>MPSSLLGAAMPASTSAAALQEALENAGRLIDRQLQEDRMYPDLSELLMVSAPNNPTVSGMSDMDYPLQGPGLLSVPNLPEISSIRRVPLPPELVEQFGHMQCNCMMGVFPPISRAWLTIDSDIFMWNYEDGGDLAYFDGLSETILAVGLVKPKAGIFQPHVRHLLVLATPVDIVILGLSYANLQTGSGVLNDSLSGGMQLLPDPLYSLPTDNTYLLTITSTDNGRIFLAGKDGCLYEVAYQAEAGWFSQRCRKINHSKSSLSFLVPSLLQFTFSEDDPILQIAIDNSRNILYTRSEKGVIQVYDLGQDGQGMSRVASVSQNAIVSAAGNIARTIDRSVFKPIVQIAVIENSESLDCQLLAVTHAGVRLYFSTCPFRQPLARPNTLTLVHVRLPPGFSASSTVEKPSKVHRALYSKGILLMAASENEDNDILWCVNHDTFPFQKPMMETQMTAGVDGHSWALSAIDELKVDKIITPLNKDHIPITDSPVVVQQHMLPPKKFVLLSAQGSLMFHKLRPVDQLRHLLVSNVGGDGEEIERFFKLHQEDQACATCLILACSTAACDREVSAWATRAFFRYGGEAQMRFPTTLPPPSNVGPILGSPVYSSSPVPSGSPYPNPSFLGTPSHGIQPPAMSTPVCALGNPATQATNMSCVTGPEIVYSGKHNGICIYFSRIMGNIWDASLVVERIFKSGNREITAIESSVPCQLLESVLQELKGLQEFLDRNSQFAGGPLGNPNTTAKVQQRLIGFMRPENGNPQQMQQELQRKFHEAQLSEKISLQAIQQLVRKSYQALALWKLLCEHQFTIIVAELQKELQEQLKITTFKDLVIRDKELTGALIASLINCYIRDNAAVDGISLHLQDICPLLYSTDDAICSKANELLQRSRQVQNKTEKERMLRESLKEYQKISNQVDLSNVCAQYRQVRFYEGVVELSLTAAEKKDPQGLGLHFYKHGEPEEDIVGLQAFQERLNSYKCITDTLQELVNQSKAAPQSPSVPKKPGPPVLSSDPNMLSNEEAGHHFEQMLKLSQRSKDELFSIALYNWLIQVDLADKLLQVASPFLEPHLVRMAKVDQNRVRYMDLLWRYYEKNRSFSNAARVLSRLADMHSTEISLQQRLEYIARAILSAKSSTAISSIAADGEFLHELEEKMEVARIQLQIQETLQRQYSHHSSVQDAVSQLDSELMDITKLYGEFADPFKLAECKLAIIHCAGYSDPILVQTLWQDIIEKELSDSVTLSSSDRMHALSLKIVLLGKIYAGTPRFFPLDFIVQFLEQQVCTLNWDVGFVIQTMNEIGVPLPRLLEVYDQLFKSRDPFWNRMKKPLHLLDCIHVLLIRYVENPSQVLNCERRRFTNLCLDAVCGYLVELQSMSSSVAVQAITGNFKSLQAKLERLH[6x];>[4x]MDTEGFGELLQQAEQLAAETEGISELPHVERNLQEIQQAGERLRSRTLTRTSQETADVKASVLLGSRGLDISHISQRLESLSAATTFEPLEPVKDTDIQGFLKNEKDNALLSAIEESRKRTFGMAEEYHRESMLVEWEQVKQRILHTLLASGEDALDFTQESEPSYISDVGPPGRSSLDNIEMAYARQIYIYNEKIVNGHLQPNLVDLCASVAELDDKSISDMWTMVKQMTDVLLTPATDALKNRSSVEVRMEFVRQALAYLEQSYKNYTLVTVFGNLHQAQLGGVPGTYQLVRSFLNIKLPAPLPGLQDGEVEGHPVWALIYYCMRCGDLLAASQVVNRAQHQLGEFKTWFQEYMNSKDRRLSPATENKLRLHYRRALRNNTDPYKRAVYCIIGRCDVTDNQSEVADKTEDYLWLKLNQVCFDDDGTSSPQDRLTLSQFQKQLLEDYGESHFTVNQQPFLYFQVLFLTAQFEAAVAFLFRMERLRCHAVHVALVLFELKLLLKSSGQSAQLLSHEPGDPPCLRRLNFVRLLMLYTRKFESTDPREALQYFYFLRDEKDSQGENMFLRCVSELVIESREFDMILGKLENDGSRKPGVIDKFTSDTKPIINKVASVAENKGLFEEAAKLYDLAKNADKVLELMNKLLSPVVPQISAPQSNKERLKNMALSIAERYRAQGISANKFVDSTFYLLLDLITFFDEYHSGHIDRAFDIIERLKLVPLNQESVEERVAAFRNFSDEIRHNLSEVLLATMNILFTQFKRLKGTSPSSSSRPQRVIEDRDSQLRSQARTLITFAGMIPYRTSGDTNARLVQMEVLMN;>[2x]MATPLAVNSAASLWGPYKDIWHKVGNALWRRQPEAVHLLDKILKKHKPDFISLFKNPPKNVQQHEKVQKASTEGVAIQGQQGTRLLPEQLIKEAFILSDLFDIGELAAVELLLAGEHQQPHFPGLTRGLVAVLLYWDGKRCIANSLKALIQSRRGKTWTLELSPELASMTTRFTDELMEQGLTYKVLTLVSQIDVNNEFEKLQRERGLGSEKHRKEVSDLIKECRQSLAESLFAWACQSPLGKEDTLLLIGHLERVTVEANGSLDAVNLALLMALLYCFDISFIEQSTEERDDMIHQLPLLTEKQYIATIHSRLQDSQLWKLPGLQATVRLAWALALRGISQLPDVTALAEFTEADEAMAELAIADNVFLFLMESVVVSEYFYQEEFYIRRVHNLITDFLALMPMKVKQLRNRADEDARMIHMSMQMGNEPPISLRRDLEHLMLLIGELYKKNPFHLELALEYWCPTEPLQTPTIMGSYLGVAHQRPPQRQVVLSKFVRQMGDLLPPTIYIPYLKMLQGLANGPQCAHYCFSLLKVNGSSHVENIQGAGGSPVSWEHFFHSLMLYHEHLRKDLPSADSVQYRHLPSRGITQKEQDGLIAFLQLTSTIITWSENARLALCEHPQWTPVVVILGLLQCSIPPVLKAELLKTLAAFGKSPEIAASLWQSLEYTQILQTVRIPSQRQAIGIEVELNEIESRCEEYPLTRAFCQLISTLVESSFPSNLGAGLRPPGFDPYLQFLRDSVFLRFRTRAYRRAAEKWEVAEVVLEVFYKLLRDYEPQLEDFVDQFVELQGEEIIAYKPPGFSLMYHLLNESPMLELALSLLEEGVKQLDTYAPFPGKKHLEKAVQHCLALLNLTLQKENLFMDLLRESQLALIVCPLEQLLQGINPRTKKADNVVNIARYLYHGNTNPELAFESAKILCCISCNSNIQIKLVGDFTHDQSISQKLMAGFVECLDCEDAEEFVRLEEGSELEKKLVAIRHETRIHILNLLITSLECNPPNLALYLLGFELKKPVSTTNLQDPGVLGCPRTCLHAILNILEKGTEGRTGPVAVRESPQLAELCYQVIYQLCACSDTSGPTMRYLRTSQDFLFSQLQYLPFSNKEYEISMLNQMSWLMKTASIELRVTSLNRQRSHTQRLLHLLLDDMPVKPYSDGEGGIEDENRSVSGFLHFDTATKVRRKILNILDSIDFSQEIPEPLQLDFFDRAQIEQVIANCEHKNLRGQTVCNVKLLHRVLVAEVNALQGMAAIGQRPLLMEEISTVLQYVVGRNKLLQCLHAKRHALESWRQLVEIILTACPQDLIQAEDRQLIIRDILQDVHDKILDDEAAQELMPVVAGAVFTLTAHLSQAVLTEQKETSVLGPAEAHYAFMLDSCFTSPPPEENPLVGFASIGDSSLYIILKKLLDFILKTGGGFQRVRTHLYGSLLYYLQIAQRPDEPDTLEAAKKTMWERLTAPEDVFSKLQRENIAIIESYGAALMEVVCRDACDGHEIGRMLALALLDRIVSVDKQQQWLLYLSNSGYLKVLVDSLVEDDRTLQSLLTPQPPLLKALYTYESKMAFLTRVAKIQQGALELLRSGVIVRLAQCQVYDMRPETDPQSMFGMRDPPMFIPTPVDRYRQILLPALQLCQVILTSSMAQHLQAAGQVLQFLISHSDTIQAILRCQDVSAGSLQELALLTGIISKAALPGILSELDVDVNEGSLMELQGHIGRFQRQCLGLLSRFGGSDRLRQFKFQDDNVEGDKVSKKDEIELAMQQICANVMEYCQSLMLQSSPTFQHAVCLFTPSLSETVNRDGPRQDTQAPVVPYWRLPGLGIIIYLLKQSANDFFSYYDSHRQSVSKLQNVEQLPPDEIKELCQSVMPAGVDKISTAQKYVLARRRLVKVINNRAKLLSLCSFIIETCLFILWRHLEYYLLHCMPTDSQDSLFASRTLFKSRRLQDSFASETNLDFRSGLAIVSQHDLDQLQADAINAFGESLQKKLLDIEGLYSKVRSRYSFIQALVRRIRGLLRISRN;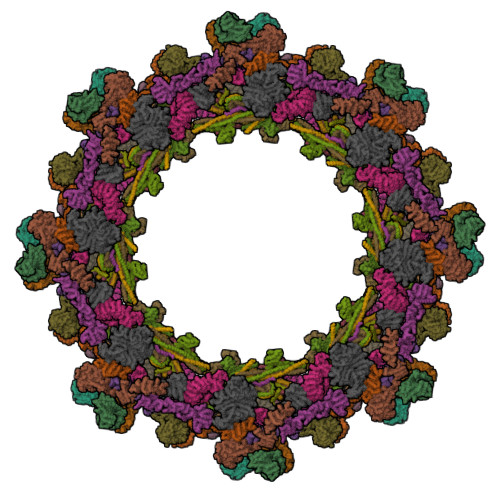>[4x]MAFNFGAPSGTSGTAAATAAPAGGFGGFGTTSTTAGSAFSFSAPTNTGTTGLFGGTQNKGFGFGTGFGTTTGTSTGLGTGLGTGLGFGGFNTQQQQQTTLGGLFSQPTQAPTQSNQLINTASALSAPTLLGDERDAILAKWNQLQAFWGTGKGYFNNNIPPVEFTQENPFCRFKAVGYSCMPSNKDEDGLVVLVFNKKETEIRSQQQQLVESLHKVLGGNQTLTVNVEGTKTLPDDQTEVVIYVVERSPNGTSRRVPATTLYAHFEQANIKTQLQQLGVTLSMTRTELSPAQIKQLLQNPPAGVDPIIWEQAKVDNPDSEKLIPVPMVGFKELLRRLKVQDQMTKQHQTRLDIISEDISELQKNQTTSVAKIAQYKRKLMDLSHRTLQVLIKQEIQRKSGYAIQADEEQLRVQLDTIQGELNAPTQFKGRLNELMSQIRMQNHFGAVRSEERYYIDADLLREIKQHLKQQQEGLSHLISIIKDDLEDIKLVEHGLNETIHIRGGVFS;>[4x]MSTGFSFGSGTLGSTTVAAGGTSTGGVFSFGTGASSNPSVGLNFGNLGSTSTPATTSAPSSGFGTGLFGSKPATGFTLGGTNTGIATTITTGLTLGTPATTSAATTGFSLGFNKPAASATPFALPITSTSASGLTLSSALTSTPAASTGFTLNNLGGTTATTTTASTGLSLGGALAGLGGSLFQSTNTGTSGLGQNALGLTLGTTAATSTAGNEGLGGIDFSSSSDKKSDKTGTRPEDSKALKDENLPPVICQDVENLQKFVKEQKQVQEEISRMSSKAMLKVQEDIKALKQLLSLAANGIQRNTLNIDKLKIETAQELKNAEIALRTQKTPPGLQHEYAAPADYFRILVQQFEVQLQQYRQQIEELENHLATQANNSHITPQDLSMAMQKIYQTFVALAAQLQSIHENVKVLKEQYLGYRKMFLGDAVDVFETRRAEAKKWQNTPRVTTGPTPFSTMPNAAAVAMAATLTQQQQPATGPQPSLGVSFGTPFGSGIGTGLQSSGLGSSNLGGFGTSSGFGCSTTGASTFGFGTTNKPSGSLSAGFGSSSTSGFNFSNPGITASAGLTFGVSNPASAGFGTGGQLLQLKKPPAGNKRGKR;>[4x]MSGFNFGGTGAPTGGFTFGTAKTATTTPATGFSFSTSGTGGFNFGAPFQPATSTPSTGLFSLATQTPATQTTGFTFGTATLASGGTGFSLGIGASKLNLSNTAATPAMANPSGFGLGSSNLTNAISSTVTSSQGTAPTGFVFGPSTTSVAPATTSGGFSFTGGSTAQPSGFNIGSAGNSAQPTAPATLPFTPATPAATTAGATQPAAPTPTATITSTGPSLFASIATAPTSSATTGLSLCTPVTTAGAPTAGTQGFSLKAPGAASGTSTTTSTAATATATTTSSSSTTGFALNLKPLAPAGIPSNTAAAVTAPPGPGAAAGAAASSAMTYAQLESLINKWSLELEDQERHFLQQATQVNAWDRTLIENGEKITSLHREVEKVKLDQKRLDQELDFILSQQKELEDLLSPLEELVKEQSGTIYLQHADEEREKTYKLAENIDAQLKRMAQDLKDIIEHLNTSGAPADTSDPLQQICKILNAHMDSLQWIDQNSALLQRKVEEVTKVCEGRRKEQERSFRITFD;>[2x]MAAAAGGPCVRSSRELWTILLGRSALRELSQIEAELNKHWRRLLEGLSYYKPPSPSSAEKVKANKDVASPLKELGLRISKFLGLDEEQSVQLLQCYLQEDYRGTRDSVKTVLQDERQSQALILKIADYYYEERTCILRCVLHLLTYFQDERHPYRVEYADCVDKLEKELVSKYRQQFEELYKTEAPTWETHGNLMTERQVSRWFVQCLREQSMLLEIIFLYYAYFEMAPSDLLVLTKMFKEQGFGSRQTNRHLVDETMDPFVDRIGYFSALILVEGMDIESLHKCALDDRRELHQFAQDGLICQDMDCLMLTFGDIPHHAPVLLAWALLRHTLNPEETSSVVRKIGGTAIQLNVFQYLTRLLQSLASGGNDCTTSTACMCVYGLLSFVLTSLELHTLGNQQDIIDTACEVLADPSLPELFWGTEPTSGLGIILDSVCGMFPHLLSPLLQLLRALVSGKSTAKKVYSFLDKMSFYNELYKHKPHDVISHEDGTLWRRQTPKLLYPLGGQTNLRIPQGTVGQVMLDDRAYLVRWEYSYSSWTLFTCEIEMLLHVVSTADVIQHCQRVKPIIDLVHKVISTDLSIADCLLPITSRIYMLLQRLTTVISPPVDVIASCVNCLTVLAARNPAKVWTDLRHTGFLPFVAHPVSSLSQMISAEGMNAGGYGNLLMNSEQPQGEYGVTIAFLRLITTLVKGQLGSTQSQGLVPCVMFVLKEMLPSYHKWRYNSHGVREQIGCLILELIHAILNLCHETDLHSSHTPSLQFLCICSLAYTEAGQTVINIMGIGVDTIDMVMAAQPRSDGAEGQGQGQLLIKTVKLAFSVTNNVIRLKPPSNVVSPLEQALSQHGAHGNNLIAVLAKYIYHKHDPALPRLAIQLLKRLATVAPMSVYACLGNDAAAIRDAFLTRLQSKIEDMRIKVMILEFLTVAVETQPGLIELFLNLEVKDGSDGSKEFSLGMWSCLHAVLELIDSQQQDRYWCPPLLHRAAIAFLHALWQDRRDSAMLVLRTKPKFWENLTSPLFGTLSPPSETSEPSILETCALIMKIICLEIYYVVKGSLDQSLKDTLKKFSIEKRFAYWSGYVKSLAVHVAETEGSSCTSLLEYQMLVSAWRMLLIIATTHADIMHLTDSVVRRQLFLDVLDGTKALLLVPASVNCLRLGSMKCTLLLILLRQWKRELGSVDEILGPLTEILEGVLQADQQLMEKTKAKVFSAFITVLQMKEMKVSDIPQYSQLVLNVCETLQEEVIALFDQTRHSLALGSATEDKDSMETDDCSRSRHRDQRDGVCVLGLHLAKELCEVDEDGDSWLQVTRRLPILPTLLTTLEVSLRMKQNLHFTEATLHLLLTLARTQQGATAVAGAGITQSICLPLLSVYQLSTNGTAQTPSASRKSLDAPSWPGVYRLSMSLMEQLLKTLRYNFLPEALDFVGVHQERTLQCLNAVRTVQSLACLEEADHTVGFILQLSNFMKEWHFHLPQLMRDIQVNLGYLCQACTSLLHSRKMLQHYLQNKNGDGLPSAVAQRVQRPPSAASAAPSSSKQPAADTEASEQQALHTVQYGLLKILSKTLAALRHFTPDVCQILLDQSLDLAEYNFLFALSFTTPTFDSEVAPSFGTLLATVNVALNMLGELDKKKEPLTQAVGLSTQAEGTRTLKSLLMFTMENCFYLLISQAMRYLRDPAVHPRDKQRMKQELSSELSTLLSSLSRYFRRGAPSSPATGVLPSPQGKSTSLSKASPESQEPLIQLVQAFVRHMQR> MRHYDCKNYINLDCEKGLCALTKGMVPIDGEGSEACPNFKPAEKCGNCKNFCNPDKYGLGTCTGLEKENWAYATCGASACP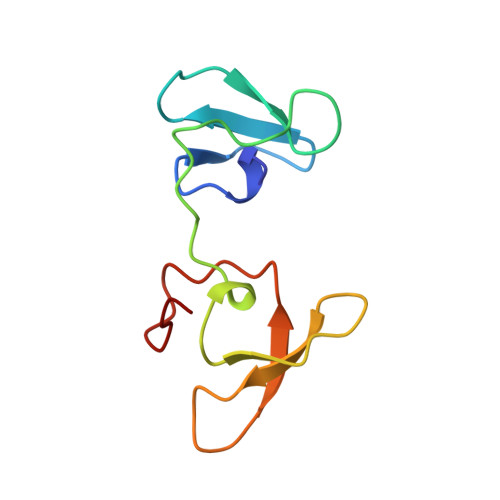SYKAE>SNAMTEINKIIHKKTFDIAWGDMDALGHVNNARYFDYFQEARIDWLRELDIKMTGQTGPVVIHVACTFLKPIVYPATVTIHS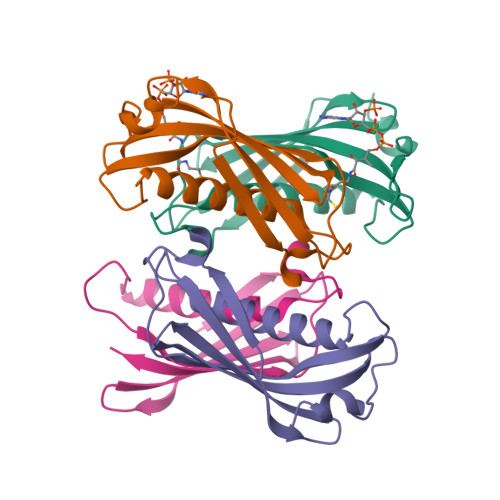KVNSLGNSSMIMDHDLYQEETLMAQGVSKIVWIDYTQNKSVPLPDIIRNLV[8x]>[2x]MIELRNLTKWYPTPHGRRYVFRNLNFRFPDDVSIGLIGRNGAGKSTLMRLLGGIEAPNEGEVVTDVSISWPVGLSGGFQGSLTARENVKFVCRIYGTSHEDMLRKVRFVEEFAEIGEHFDLPMKTYSSGMRSRVAFGLSMAFDFDYYLIDEAMAVGDAQFRAKSRAVFDSRVGQANMILVSHNMNDIKEYCDVVVLVDQGQATLYEDVEAGIAAYQGSLKKAAAKPDYKDDDDK;>MGKIHLAVSERSPRVKRSPWQIQQAVLFALFLRELKTRLGGRWLGVFWVLLEPVAHIAVMTTLFSLAHRAAMPSIEYPVFLITGLIPFFMFRGLVTRLMEAIDSNRGLFAYRQVKPIDTVIARAMLEISLQSIVYLIALGTLGWLGFHFLPVRALELAGVSAVLIMLGASLGLFFAVVTNEIPQARAIVRISLLPLYFVSGVIFPVHTIPPQYLPLLQLNPVLHLIELSRASFFPQYRVLQGINLAYPAGFALLSLFLALMLYRLRRHQLASVV[2x];>MGKIHMKLVSRLTAKRLQWALVYLPMLVATVYFLVFSADRYVSESVITVRQTSSNAPTGGMSGAALLLAGLTPASREDTCYLQTYIHSMGLLQKLDQQLKLREHFGTPLRDPLFRLWGGTSQEWFLEYYRSRVEVLMDDICGLLTVRVQGFEPEFAQALNRAILEESERFVNELSHRMAREQGQFAEAELERATARLQEAKRQLIAFQAKHKLLDPLAQAQATGTLTAELQAALTRQEAELRNALTYLNEDSYQVKALRSQINALRQQIDEERLRATAGKNGDRINAVAAEFHDLQLQVGFAEDAYKLALAAVESARIEATRKLKSLVVVEPPVLPEIAEYPRRWYNLATLLVVCCLIYGVVSLVVATIRDHQDGSGSGSHHHHHHHHHH[8x]

CPS secretion is mediated by an ABC transporter containing KpsT and KpsM as its nucleotide-binding domain (NBD) and transmembrane domain, respectively. The transporter partners with the periplasmic and inner-membrane-anchored KpsE subunit, a class-3 polysaccharide co-polymerase (PCP), as well as with KpsD, which is assumed to form an outer-membrane pore. The KpsMT transporter is surrounded by a cage of eight KpsE subunits extending about 80 Å into the periplasm. Cryo-electron microscopy analyses of the KpsMT–KpsE complex in six different states reveal a KpsE-encaged ABC transporter, rigid-body conformational rearrangements of KpsMT during ATP hydrolysis and recognition of a glycolipid inside a membrane-exposed electropositive canyon.

In a nucleotide-free state, our cryo-EM analyses resolve two apo KpsMT conformations (Apo 1 and Apo 2). In the Apo 2 state, the NBDs are closer together and slightly shifted against each other. A similar arrangement has been observed in the crystal structure of the isolated Wzt NBD dimer of the O-antigen ABC transporter. Accordingly, the KpsM subunits move towards each other by about 12 Å as compared to the Apo 1 state, reducing the separation of the membrane-embedded subunits and narrowing the electropositive canyon.> HHMNPNAT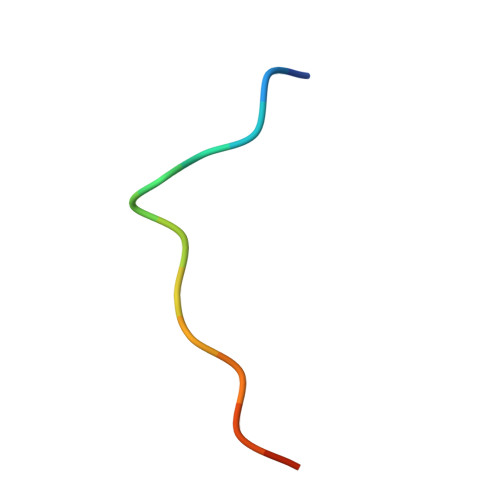EFMPGR(1~{S},4~{R},5~{S})-7,7-bis(chloranyl)-6,6-bis(oxidanyl)-2$l^{4}-thiabicyclo[3.2.0]hept-2-ene-4-carboxylic acid | C7 H8 Cl2 O4 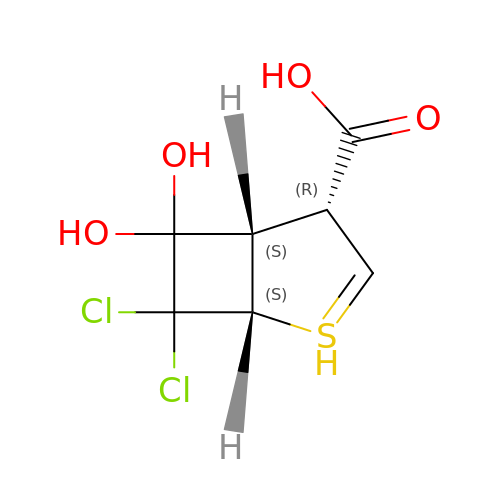S | CYWQDVFNRSXKKZ-JJYYJPOSSA-N>[2x]MTAASLDPTAFSLDAASLAARLDAVFDQALRERRLVGAVAIVARHGEILYRRAQGLADREAGRPMREDTLFRLASVTKPIVALAVLRLVARGELALDAPVTRWLPEFRPRLADGSEPLVTIHHLLTHTSGLGYWLLEGAGSVYDRLGISDGIDLRDFDLDENLRRLASAPLSFAPGSGWQYSLALDVLGAVVERATGQPLAAAVDALVAQPLGMRDCGFVSAEPERFAVPYHDGQPEPV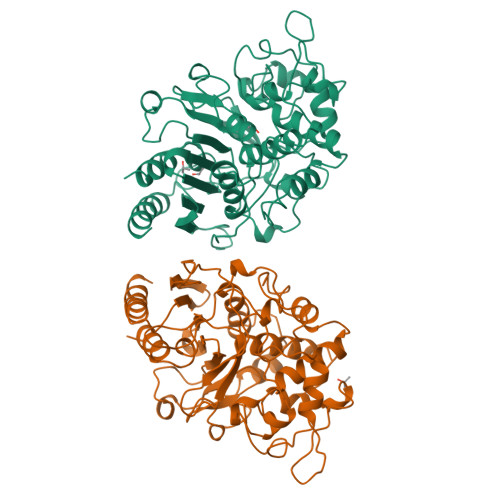RMRDGIEVPLPEGHGAAVRFAPSRVFEPGAYPSGGAGMYGSADDVLRALEAIRANPGFLPETLADAARRDQAGVGAETRGPGWGFGYLSAVLDDPAAAGTPQHAGTLQWGGVYGHSWFVDRALGLSVLLLTNTAYEGMSGPLTIALRDAVYAR The KEOPS complex, which is conserved across archaea and eukaryotes, is composed of four core subunits; Pcc1, Kae1, Bud32 and Cgi121. Kae1 catalyzes the universal and essential tRNA modification N6-threonylcarbamoyl adenosine, but the precise roles of all other KEOPS subunits remain an enigma. Here we show using structure-guided studies that Cgi121 recruits tRNA to KEOPS by binding to its 3’ CCA tail. A composite model of KEOPS bound to tRNA reveals that all KEOPS subunits form an extended tRNA-binding surface that we have validated in vitro and in vivo to mediate the interaction with the tRNA substrate and its modification.

Overall, mjCgi121 engaged the tRNA in a manner that sterically caps its free 5′ and 3′ termini. mjCgi121 contacts the tRNA through an extensive surface (1162 Å2) involving helices-α1, -α3, and -α4, in agreement with the NMR analysis. Contacts with the tRNA are directed largely at the universal 3′ CCA tail (C74, C75, and A76) (see Supplementary Fig. 2b for an unbiased electron density map), and to a lesser degree at G73. The mjCgi121–tRNA interface involves a mixture of hydrophobic, hydrogen-bonding and salt interactions. The base of A76 engages a deep hydrophobic pocket formed by Gly80 and the side chains of Phe21, Met60, and Ile76. The ribose 3′ hydroxyl group of A76 is tightly packed against Cgi121, which may disfavor the binding of aminoacylated tRNAs. The base of C75 forms hydrophobic contacts with the side chains of Lys56, Met60, and Ile72. The base of C74 forms hydrophobic contacts with the Ile72 side chain, and a hydrogen-bond with the peptide backbone of Ile72. In conclusion, these crystallographic analyses revealed a binding mode of mjCgi121 to tRNA that is counter-intuitively directed at a universal element of tRNAs that is maximally distant (>65 Å) from the A37 site of t6A modification.

> GAMDPMIIRGIRGARINNEIFNLGLKFQILNADVVATKKHVLHAINQAKTKKPIAKSFWMEILVRASGQRQIHEAIKIIGAKDGNVCLICEDEETFRKIYELIGGEIDDSVLEINEDKERLIREIFKIRGFGNVVERVLEKIALIELKKE> MNSEYDYLFKLLLIGNSGVGKSCLLLRFSDDTYTNDYISTIGVDFKIKTVELDGKTVKLQIWDTAGQERFRTITSSYYRGSHGIIIVYDVTDQESFNGVKMWLQEIDRYATSTVLKLLVGNKCDLKDKRVVEYDVAKEFADANKMPFLETSALDSTNVEDAFLTMARQIKESMSQQNLNE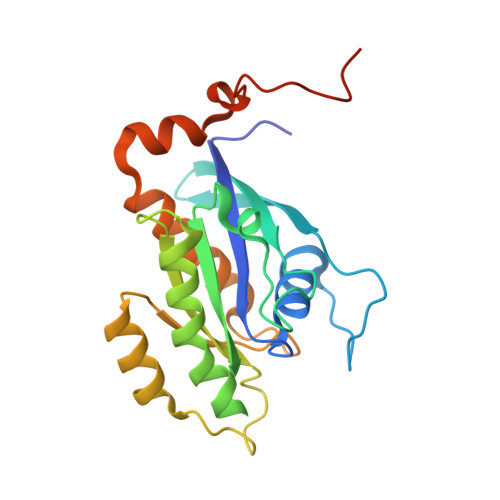TTQKKEDKGNVNLKGQSLTNTGGCCC> MGSSHHHHHHSSGENLYFQGHHMGKKLSLIDFNEIYNEENLITRANPIENHEFSDDGIYSERIFGSYNEDDDDKDIDTIGWINIEPYYIINPILFTIIKKCIPSINKIINYQQSIDQNGENIDLTEEIGEDDYIGLVKFKDNFDDLLEKYTDKKKYQKEYDFLIENHDKIFINKLPVFSHKLRPATLLTGSKGKVLAFDEINNYYNFVIEYINQINEGVVSDDSIDLLLLPLLYNMQFYANNILTRIISEYLRGKKGFLRKNIMGSRINFSARNVITPLIGHPIDEVAMPYKTFAELYKFQLINLISKVKGINYNEALKFWEKGILGFNQELYNYMEELITKTKGGCTFLLNRNPTIS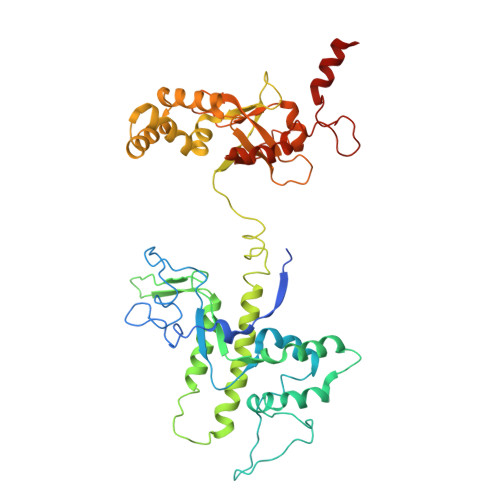IGSILYLKIGLIKKDYKDLTLGISNNLLSALSGDYDGDVLNIIPVFDNKMKEHFSLLSPQNFLVDRNNGRFNGDFDLQKDQILGIFILNN>[2x]GSHMSSGYPGVSWNKRMCAWLAFF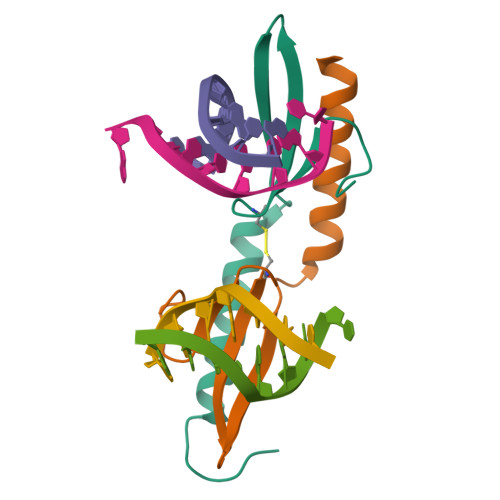YDGASRRSRTFHPKHFNMDKEKARLAAVEFMKTVENNGRKKLEPGGSQFIVTD>TSTKRFTCPEESEASNCSCEEFPSKTHFYCPDFNPTLYVDVEDRMRVDFKCYDEPHDFKSLPNLAIGSVKLLTVVDCVLDDDRPILESFKFLEVADVRSFVYNNHENGIRYNAKYFEGMEQLENLTLARGVVSIDRDTFSGFLNLKRLTIEHNKLNLQPGTFEALSNLTYLGLVYNGLNEIQPGLFDGLESLEALSLSYNDIKSLSAGSFNGLSSLRMLNLRVNKIESFDANTFASLKELSRLEITLNPFVSLPRGLFSENKKLKTLILTNNRKLVTLPEELLANLKELTVVNLSHNGVGNLPESLLSGSSGIIELNLGYNRLNSLPEELLSDQPQLQVLNLDHNQLESIPDYFLERNVELQTLYLSHNRLRSLSEKAFTKLKNLKELHLENNQLQTIPQFLFSGTPKLEEIYMQNNQLALHANSFINEELSIADNDNTPFQVLQKLRILHLRNNSISTIFQDWYINNLEMQSLDLSFNKLPGLSYTQLQFQSNITLNLSNNEISQVLLIDDLDLQPYQRINVDLNHNPLNCNCNALKFIQLIQSKAEHGLQFNVDQLRCSEPPNLLDATMDQLQTKDLLCDFES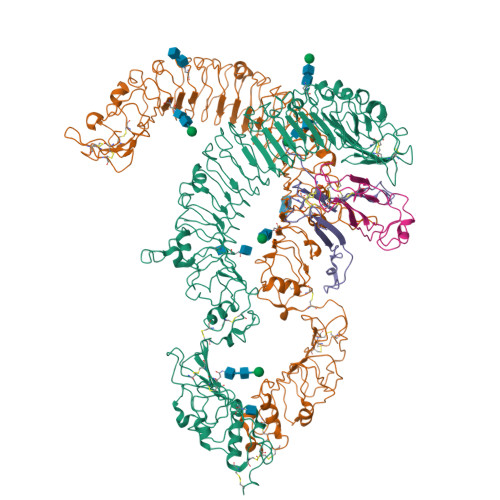ADDCPKDCQCAMRLLDHTVIVNCSGRGLTEFPDLPIPSQLHEDFNALEVHVENNRLTKLPNLTKHNEITQLYARNNSIQNLLPHNIPSKLRIIDLSQNLLKMIDDSTLAQINRSSHLETIRLSQNQWLCDCPASSFLIFVQQNSRLISDMSAIRCHPSGKSLDSITVNELCFEDYTTENLYFQ[2x];>[2x]SDTANAPFLCESEQLLIHPKEELSRNNSMVWIVNTKDYKQGVRIEKCLKRQLGKPCNFCDADTECKQLFHYRTLVAVDKVTKKPYKEQVLLPSCCKCAKILSTGWSHPQFEK>MGHHHHHHDDKQWERFLVPYRQAVEELKVKLKGIRTLYEYEDDHSPIEFVTGRVKPVASILEKARRKSIPLHEIETMQDIAGLRIMCQFVDDIQIVKEMLFARKDFTVVDQRDYIAEHKESGYRSYHLVVLYPLQTVSGEKHVLVEIQIRTLAMNFWATIEHSLNYKYSGNIPEKVKLRLQRASEA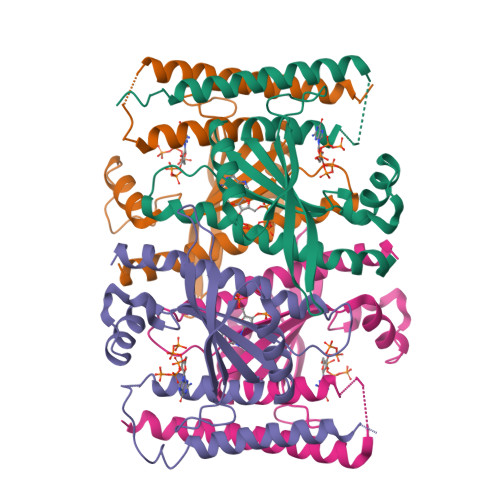ASRLDEEMSEIRGEVQEAQAAFSRKKKGSEQQ[8x]> MANHYLRIFQQPKSAILLILGFASGLPLALTSGTLQAWMTVENIDLKTIGFFSLVGQAYVFKFLWSPVMDRYTPPFLGRRRGWLVTTQILLLIAIAAMGFLEPGTQLRWMAALAVVIAFCSASQDIVFDAWKTDVLPAEERGTGAAISVLGYRLGMLVSGGLALWMADKWLGWQGMYWLMAALLVPCIIATLLAPEPSDVVPVPRTLEQAVVAPLRDFFGRN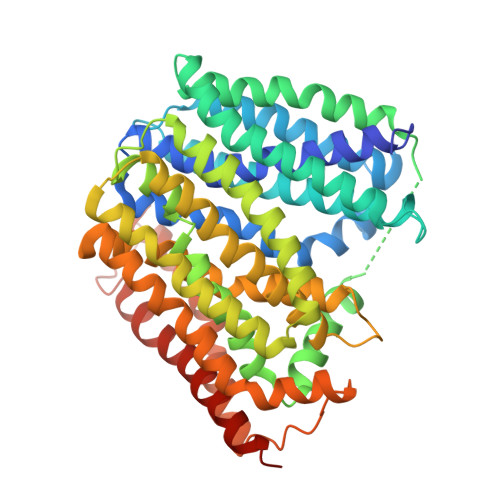NAWLILLLIVLYKLGDAFAMSLTTTFLIRGVGFDAGEVGMVNKTLGLIATIIGALYGGVLMQRLSLFRALLIFGILQGVSNAGYWLLSITDKHLMSMAVAVFFENLCGGMGTAAFVALLMTLCNKSFSATQFALLSALSAVGRVYVGPIAGWFVEAHGWPTFYLFSVFAAVPGILLLLICRKTLEYTQQTESFMMRRHFSGAYQFALYLLLLGCLLLALWLIMLALNAIDYTSFSFLAGLLEVAALIAIAGVLLGAILDYLALRRTEEHKLA>MSNQYGDKNLKIFSLNSNPELAKEIADIVGVQLGKCSVTRFSDGEVQINIEESIRGCDCYIIQSTSDPVNEHIMELLIMVDALKRASAKTINIVIPYYGYARQDRKARSREPITAKLFANLLETAGATRVIALDLHAPQIQGFFDIPIDHLMGVPILGEYFEGKNLEDIVIVSPDHGGVTRARKLADRLKAPIAIIDKRRPRPNVAEVMNIVGNIEGKTAILIDDIIDTAGTITLAANALVENGAKEVYACCTHPVL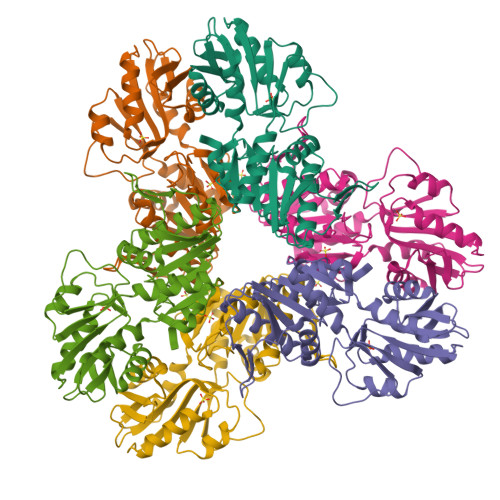SGPAVERINNSTIKELVVTNSIKLPEEKKIERFKQLSVGPLLAEAIIRVHEQQSVSYLFS[2x]> DANLLNDRVLRAMLKAEETCAPSVSYFKCVQKEVLPSMRKIVATWMLEVCEEQKCEEEVFPLAMNYLDRFLSLEPVKKSRLQLLGATCMFVASKMKETIPLTAEKLCIYTDNSIRPEELLQMELLLVNKLKWNLAAMTPH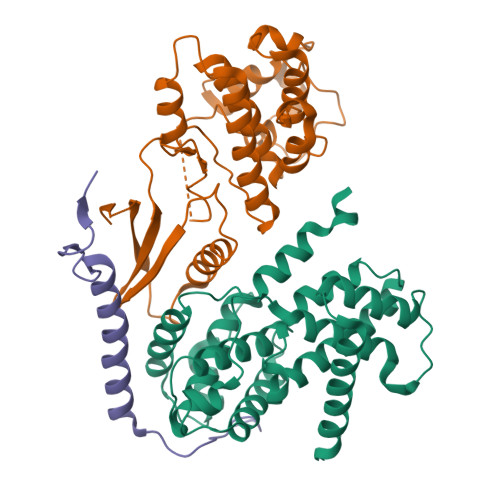DFIEHFLSKMPEAEENKQIIRKHAQTFVALCATDVKFISNPPSMVAAGSVVAAVQGLNLRSPNNFLSYYRLTRFLSRVIKCDPDCLRACQEQIEALLESSLRQAQQNMD;> GEFATSRYEPVAEIGVGAYGTVYKARDPHSGHFVALKSVRVPNGEEGLPISTVREVALLRRLEAFEHPNVVRLMDVCATSRTDREIKVTLVFEHVDQDLRTYLDKAPPPGLPAETIKDLMRQFLRGLDFLHANCIVHRDLKPENILVTSGGTVKLADFGLARIYSYQMALTPVVVTLWYRAPEVLLQSTYATPVDMWSVGCIFAEMFRRKPLFCGNSEADQLGKIFDLIGLPPEDDWPRDVSLPRGAFPPRGPRPVQSVVPEMEESGAQLLLEMLTFNPHKRISAFRALQHSYLHKDEGNPE;> GEFKPSACRNLFGPVDHEELTRDLEKHCRDMEEASQRKWNFDFQNHKPLEGKEEWQEVEKGSLPEFEERPPR> KLAFPRELRLLTPSQFTFVFQQPQRAGTPQITILGRLNSLGHPRIGLTVAKKNVRRAHE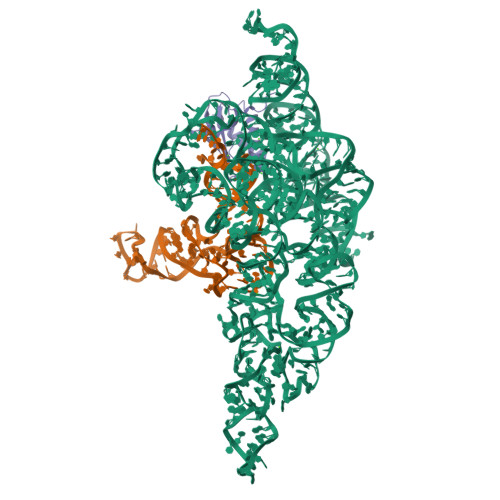RNRIKRLTRESFRLRQHELPAMDFVVVAKKGVADLDNRALSEALEKLWRRHCR> MKIKEIK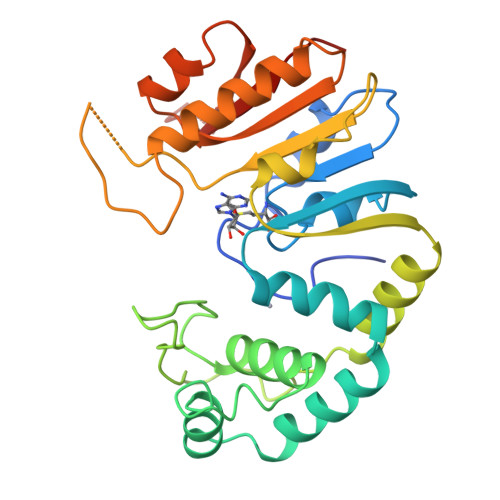KVTLQPFTKWTGGKRQLLPVIRELIPKTYNRYFEPFVGGGALFFDLAPKDAVINDFNAELINCYQQIKDNPQELIEILKVHQEYNSKEYYLDLRSADRDERIDMMSEVQRAARILYMLRVNFNGLYRVNSKNQFNVPYGRYKNPKIVDEELISAISVYINNNQLEIKVGDFEKAIVDVRTGDFVYFDPPYIPLSETSAFTSYTHEGFSFADQVRLRDAFKRLSDTGAYVMLSNSSSALVEELYKDFNIHYVEATRTNGAKSSSRGKISEIIVTNYEK>[4x]MKTRTQQIEELQKEWTQPRWEGITRPYSAEDVVKLRGSVNPECTLAQLGAAKMWRLLHGESKKGYINSLGALTGGQALQQAKAGIEAVYLSGWQVAADANLAASMYPDQSLYPANSVPAVVERINNTFRRADQIQWSAGIEPGDPRYVDYFLPIVADAEAGFGGVLNAFELMKAMIEAGAAAVHFEDQLASVKKCGHMGGKVLVPTQE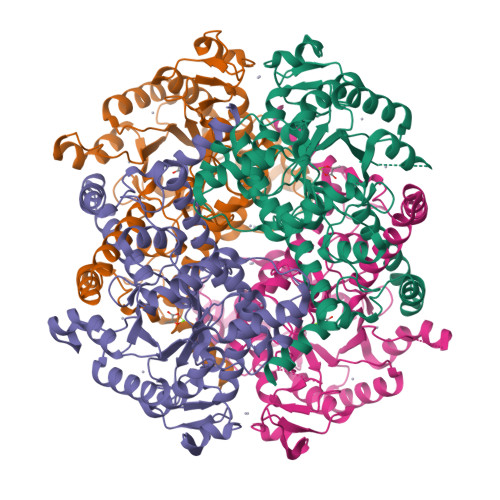AIQKLVAARLCADVTGVPTLLVARTDADAADLITSDCDPYDSEFITGERTSEGFFRTHAGIEQAISRGLAYAPYADLVWCETSTPDLELARRFAQAIHAKYPGKLLAYNCSPSFNWQKNLDDKTIASFQQQLSDMGYKFQFITLAGIHSMWFNMFDLANAYAQGEGMKHYVEKVQQPEFAAAKDGYTFVSHQQEVGTGYFDKVTTIIQGGTSSVTALTGSTEESQF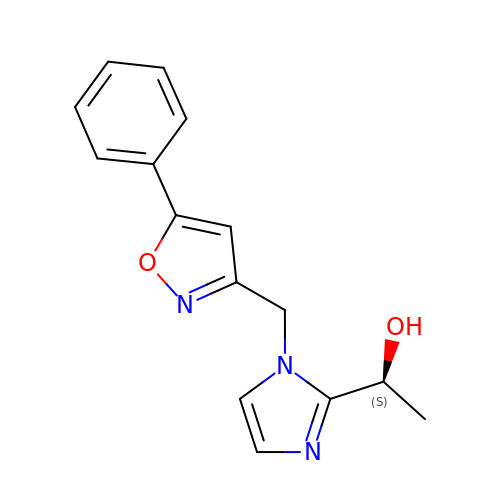(1S)-1-[1-[(5-phenyl-1,2-oxazol-3-yl)methyl]imidazol-2-yl]ethanol | C15 H15 N3 O2 | AFOXOGZPNJAOMI-NSHDSACASA-N>MFTGWSPFKYSKGNTVTFKTPDESSIAYMRFRNCVFTFTDPKGSLHSIDVTE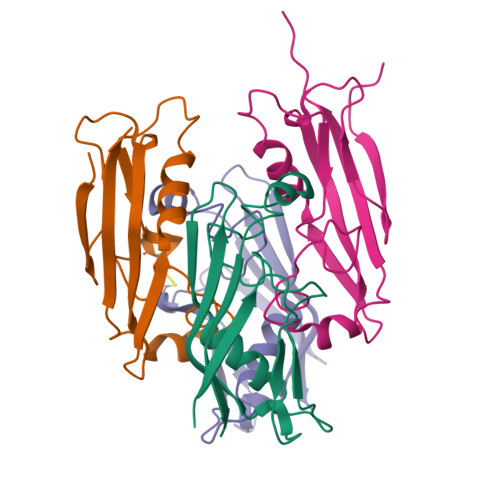VLNNMAKGFRDAQNPPSSFTLGGHCQAPLNAFSFVLPGVNDRATVATADEAKKWENCDATLTGLQRIIHHHHHH[6x]>MLSPIRTTFHNSVNIVQSSPSQTVSFAGKEYELKVIDEKTPILFQWFEPNPERYKKDEVPIVNTKQHPYLDNVTNAARIESDRMIGIFVDGDFSVNQKTAFSKLERDFENVMIIYREDVDFSMYDRKLSDIYHDIICEQRLRTEDKRDEYLLNLLEKELREISKAQDSLISMYAKKRNHAWFDFFRNLALLKAGEIFRSTYNTKNHGISFGEGCIYLDMDMILTGKLGTIYAPDGISMHVDRRNDSVNIENSAIIVN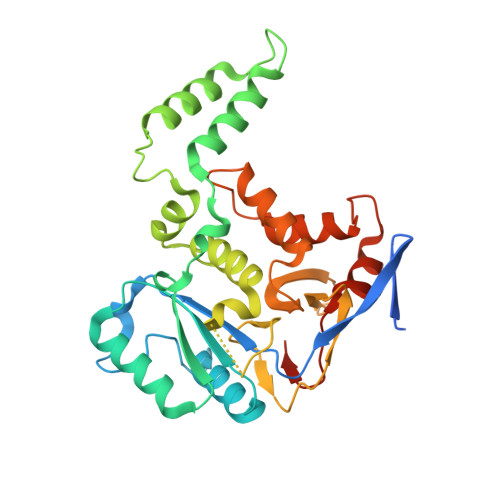RSNHPALLEGLSFMHSKVDAHPYYDGLGKGVKKYFNFTPLHNYNHFCDFIEFNHPNIIMNTSQYTCSSW[2x]MgtE is a widely distributed Mg2+ channel in both prokaryotes and eukaryotes. The bacterial MgtE channels are highly selective for Mg2+, and are involved in the maintenance of the intracellular Mg2+ concentration. The full-length structure in the presence of Mg2+ revealed that MgtE forms a homodimer, consisting of five transmembrane helices, one plug helix, and the cytosolic region composed of the N-terminal domain and the tandemly repeated CBS domains. A comparative analysis of the Mg2+-bound and Mg2+-free cytosolic domain structures, together with molecular dynamic simulations, revealed that Mg2+ binding to the cytosolic domain stabilizes the closed conformation of MgtE, suggesting a Mg2+ homeostasis mechanism in which the MgtE cytosolic domain acts as a Mg2+ sensor to regulate the Mg2+ influx.

We also determined the crystal structure of the cytosolic domain of MgtE in complex with ATP at 3.0 Å resolution. The overall structure of the cytosolic domain is essentially identical to that in the full-length MgtE structure in complex with ATP, with an RMSD value of 0.9 Å for 230 Cα atoms. Since the cytosolic domain structure was solved at a higher resolution, we describe the ATP binding by MgtE mainly based on the structure of the cytosolic domain of MgtE in complex with ATP. ATP molecules are located proximal to the subunit interface between the N domain in one subunit and the CBS domain in the neighboring subunit. While we observed the binding of Mg2+ ions to the cytosolic domain, as reported in the previous MgtE structures, the phosphate groups of ATP are 5.4 Å away from the closest Mg2+ ion in the ATP-bound structure. Therefore, ATP binding to MgtE may not be directly coupled with Mg2+ binding. The ATP molecule is exclusively recognized by the CBS domain. The adenine base of ATP is stabilized by three hydrogen bonds with the side chain of Asn203, and the main-chain carbonyl and amino groups of Val207, together with a π stacking interaction with Phe227. The ribose moiety of ATP forms two hydrogen bonds with the side chain of Asp188, while the α- and β-phosphates of ATP interact with the side chains of Tyr170 and Arg187, respectively. The phosphate groups of ATP adopt the extended conformation, and thus the three phosphate groups are exposed to the subunit interface between the N and CBS domains.

>GSHMEEKLAVSLQEALQEGDTRALREVLEEIHPQDLLALWDELKGEHRYVVLTLLPKAKAAEVLSHLSPEEQAEYLKTLPPWRLREILEELSLDDLADALQAVRKEDPAYFQRLKDLLDPRTRAEVEALARYEEDEAGGLMTPEYVAVREGMTVEEVLRFLRRAAPDAETIYYIYVVDEKGRLKGVLSLRDLIVADPRTRVAEIMNPKVVYVRTDTDQEEVARLMADYDFTVLPVVDEEGRLVGIVTVDDVLDVLEAEATEDIHKLGAVDVPDLVYSE[4x]We therefore set out to characterize two previously unstudied proteins from the shipworm symbiont Teredinibacter turnerae that were initially identified by the presence of carbohydrate binding domains appended to uncharacterized domains with probable redox functions. One of these was TERTU_3803, which contained both a CBM10 and a CBM2 domain attached to a range of distinct modules (via flexible linkers) that did not bare any sequence similarity with catalytic domains typically found within carbohydrate-active enzymes. Using a ‘module walking’ approach, we searched for other genes coding for these X-domains. This led to the identification of TERTU_2913, which lacks CBMs but contains predicted X122, X183 and X132 domains. Taken together, these sequence analyses suggested that TERTU_3803 and TERTU_2913 could have a role to play in cellulose metabolism, and furthermore that role is likely to be a redox one given the presence of cytochrome domains within their linear amino acid sequences.

In addition to our work on Ttpf08450-X173, we produced TtX122A and TtX122B, representing the X122 domains from TERTU_3803 and TERTU_2913, respectively. The electron density was readily interpretable allowing two molecules of TtX122A to be modelled in the asymmetric unit without breaks in the chain representing residues 3 to 244 of the protein coded for in our construct. Three molecules of TtX122B were present in the asymmetric unit, with chain B’s electron density most readily traced allowing modelling of residues 2 to 235 without breaks in the chain. Chains A and C had some areas that displayed more disorder, so there were breaks in the model between residues 190 and 192 in chain A and residues 162 and 165 in chain C. In addition to protein and water molecules, two magnesium ions were modelled into the electron density on each protomer in TtX122A based on coordination geometry and bond lengths [Fig. S4(a)]; these ions presumably bound from the crystallization medium. To check the oligomeric state of our TtX122 structures, PISA analysis was performed, which revealed that there were no significant molecular interfaces between protomers in the crystal for either structure, suggesting that the molecules would be expected to be monomeric in solution. Our subsequent structural analysis therefore focused on single protomers from each structure. The overall structures of TtX122A and TtX122B reveal that these domains adopt a β-jelly-roll fold [Figs. 4(a) and 4(b)].

>[2x]GGSLINFTDGFESTGVNQQPSGWGNFVGWQSNNPNNNIGQSVYALVDNTRAFTGNNSVHFKGGAAPAQIVRTLPAGLDKVYLKAMVYMSKKLGNEAGDNHEHIFGVRGNVAQADNEVRFGQIKGHVGTNEMPSDDISPPQSQWYSGPEIAADTWHCVVVEMLGGNRPYHQLHAYLDNQLIHSIDSISDWNNGGVNGNTQWLDGKLNYAFFGWHSFSNNNADVWMDDIEISDQPISCDSRELEHHHHHH>[2x]MEHKRGHVLAVPYPTQGHITPFRQFCKRLHFKGLKTTLALTTFVFNSINPDLSGPISIATISDGYDHGGFETADSIDDYLKDFKTSGSKTIADIIQKHQTSDNPITCIVYDAFLPWALDVAREFGLVATPFFTQPCAVNYVYYLSYINNGSLQLPIEELPFLELQDLPSFFSVSGSYPAYFEMVLQQFINFEKADFVLVNSFQELELHENELWSKACPVLTIGPTIPSIYLDQRIKSDTGYDLNLFESKDDSFCINWLDTRPQGSVVYVAFGSMAQLTNVQMEELASAVSNFSFLWVVRSSEEEKLPSGFLETVNKEKSLVLKWSPQLQVLSNKAIGCFLTHCGWNSTMEALTFGVPMVAMPQWTDQPMNAKYIQDVWKAGVRVKTEKESGIAKREEIEFSIKEVMEGERSKEMKKNVKKWRDLAVKSLNEGGSTDTNIDTFVSRVQSK

UGT74F1 and UGT74F2 are the enzymes responsible for the in vivo glucosylation of SA in A. thaliana. In UGT74F1, glucose is transferred to the hydroxyl of SA, creating a glucoside; in UGT74F2, glucose is transferred to the carboxylate group of SA to create a glucose ester. UGT74F2 exhibits the GT-B fold with ligands bound in the cleft between the two domains –the N-terminal domain is comprised of residues 1–245, while 246–449 make up the C-terminal domain. UDP and SA interact primarily with residues in the C- and N-terminal domain, respectively.

To identify the binding pocket of SA, UGT74F2 was co-crystallized with UDP and SA or SA analogue 2-bromobenzoic acid (2-BA). In the co-crystal of UGT74F2 with UDP and SA, the SA omit map shows clear density for a small molecule within a pocket in the acceptor binding domain. Two different conformations of SA were modeled in the omit electron density. Analysis of the crystallographic thermal parameters (B factors) of SA and surrounding protein residues support the SA conformation shown in Fig. 3c. Tyr 13, Thr 15, His 18, Phe 113, Gln 134, Tyr 180, Met 183, Met 274, Val 184, Trp 364 and Thr 365 delineate the SA binding pocket. Van der Waals interactions between the benzoic ring of SA and Phe 133, Tyr 180, Met 183, Met 274, Trp 364, and Thr 365 constrain the approximate location of SA, while the carboxylate group of SA interacts through hydrogen bonds with His 18 and Thr 15. The conserved catalytic His 18-Asp 111 dyad is below SA; there is a hydrogen bond from His 18 to the carboxylate group of SA, which is positioned 2.6 Å from the anomeric carbon of UDP-glucose. Based on the observed SA and modeled UDP-glucose, we propose a SN2 reaction for SGE formation by UGT74F2. SA carboxyl is positioned towards the anomeric carbon of UDP-glucose by hydrogen bond interactions with His 18 and Thr 15. Given the pH dependence of SGE formation and the critical role of His 18 in UGT74F2 activity, His 18 is probably protonated and forms hydrogen bond interactions both with Asp 111 and one of the oxygens of the SA carboxylate group.>MITAQAVLYTQHGEPKDVLFTQSFEIDDDNLAPNEVIVKTLGSPVNPSDINQIQGVFPSKPAKTTGFGTTEPAAPCGNEGLFEVIKVGSNVSSLEAGDWVIPSHVNFGTWRTHALGNDDDFIKLPNPAQSKANGKPNGLTINQGATISVNPLTAYLMLTHYVKLTPGKDWFIQNGGTSAVGKYASQIGKLLNFNSISVIRDRPNLDEVVASLKELGATQVITEDQNNSREFGPTIKEWIKQSGGEAKLALNCVGGKSSTGIARKLNNNGLM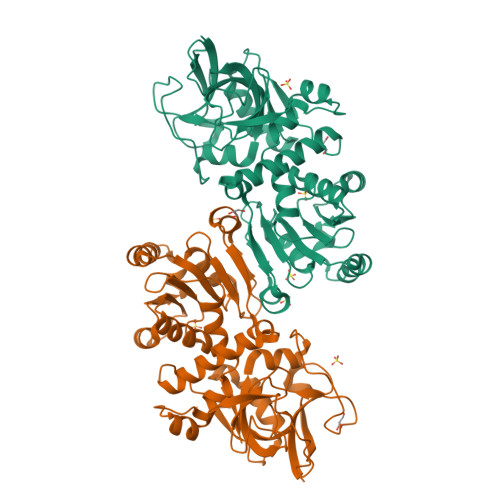LTYGGMSFQPVTIPTSLYIFKNFTSAGFEVTELLKNNKELKTSTLNQIIAWYEEGKLTDAKSIETLYDGTKPLHELYQDGVANSKDGKQLITY[2x]> GPKQKIVIKVSMPCEKSRSKAMKLVVMASGVSSVEVTGDGKDRLQVVGDGVDAACLVT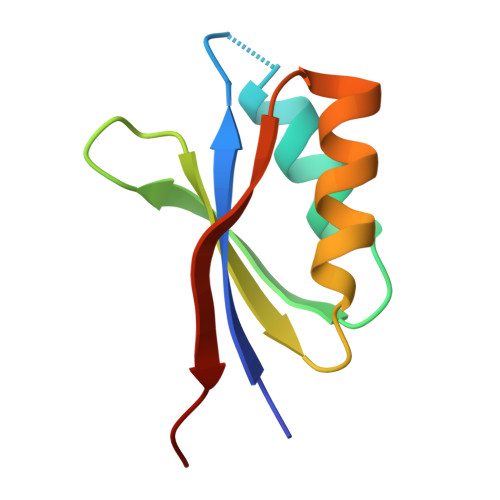CLRKKIGHAELVQVEEVKEK>[4x]MASMTGGQQMGRIQAD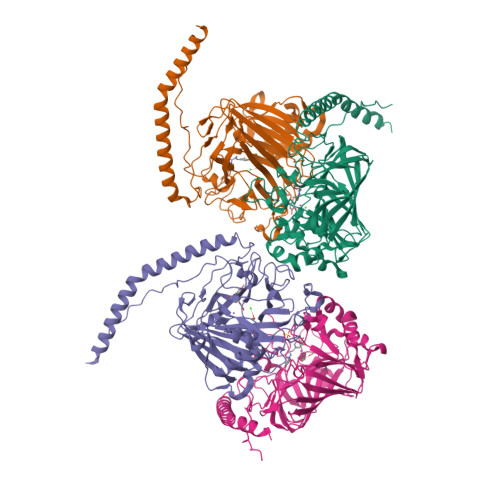YEAKLAKYQADLAKYQKDLADYPVKLKAYEDEQTSIKAALAELEKHKNEDGNLTEPSAQNLVYDLEPNANLSLTTDGKFLKASAVDDAFSKSTSKAKYDQKILQLDDLDITNLEQSNDVASSMELYGNFGDKAGWSTTVSNNSQVKWGSVLLERGQSATATYTNLQNSYCNGKKISKIVYKYTVDPKSKFQGQKVWLGIFTDPTLGVFASAYTGQVEKNTSIFIKNEFTFYDEDGKPINFDNALLSVASLNREHNSIEMAKDYSGKFVKISGSSIGEKNGMIYATDTLNFKQGEGGSRWTMYKNSQAGSGWDSSDAPNSWYGAGAIKMSGPNNYVTVGATSATNVMPVSDMPVVPGKDNTDGKKPNIWYSLNGKIRAVNVPKVTKEKPTPPVKPTAPTKPTLEHHHHHH6-fluoranyl-~{N}-(4-pyridin-2-yl-1,3-thiazol-2-yl)-1,3-benzothiazol-2-amine 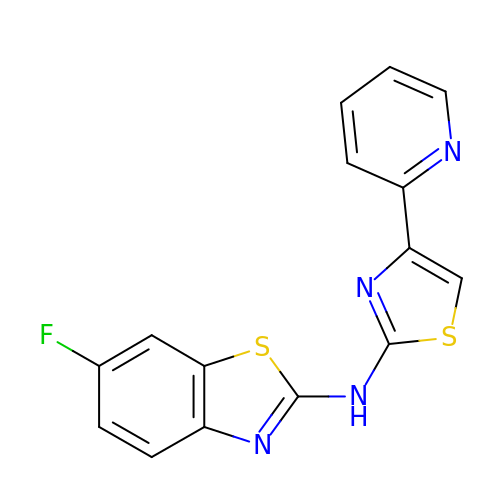| C15 H9 F N4 S2 | CKLUPEBKNDQOFT-UHFFFAOYSA-N>[2x]AECKVTVDSTDQMSFNTKDIAIDKSCKTFTVELTHSGSLPKNVMGHNLVISKEADMQPIATDGLSAGIDKQYLKDGDARVIAHTKVIG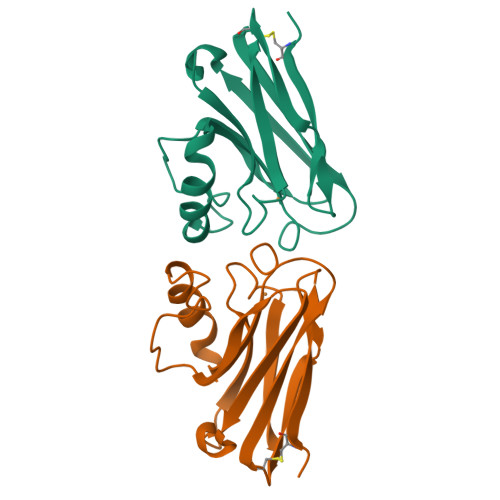AGEKDSVTFDVSKLAAGEKYGFFCSFPGHISMMKGTVTLK> TNWESLYEKALDKVEASIRKVRGVLLAYNTNIDAIKYLKREDLEKRIEKVGKEEVLRYSEELPKEIETIPQLLGSILWSIKRGKAAELLVVSREVREYMRKWGWDELRMGGQVGIMANLLGGVYGIPVIAHVPQLSELQASLFLDGPIYVPTFERGELRLIHPREFRKGE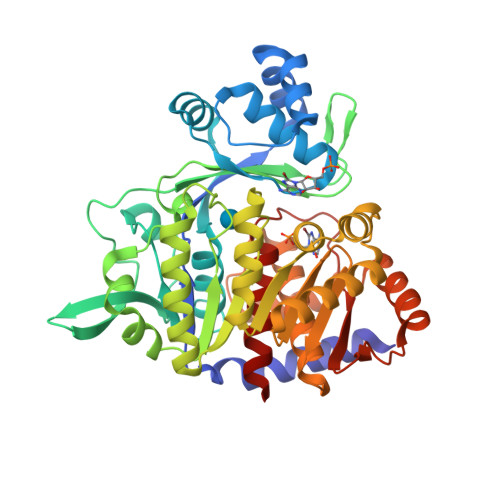EDCIHYIYEFPRNFKVLDFEAPRENRFIGAADDYNPILYVREEWIERFEEIAKRSELAIISGLHPLTQENHGKPIKLVREHLKILNDLGIRAHLEFAFTPDEVVRLEIVKLLKHFYSVGLNEVELASVVSVMGEKELAERIISKDPADPIAVIEGLLKLIKETGVKRIHFHTYGYYLALTREKGEHVRDALLFSALAAATKAMKGNIEKLSDIREGLAVPIGEQGLEVEKILEKEFSLRDGIGSIEDYQLTFIPTKVVKKPKSTVGIGDTISSSAFVSEFSLH5-(trifluoromethyl)-2,3-dihydro-1~{H}-1,4-diazepine 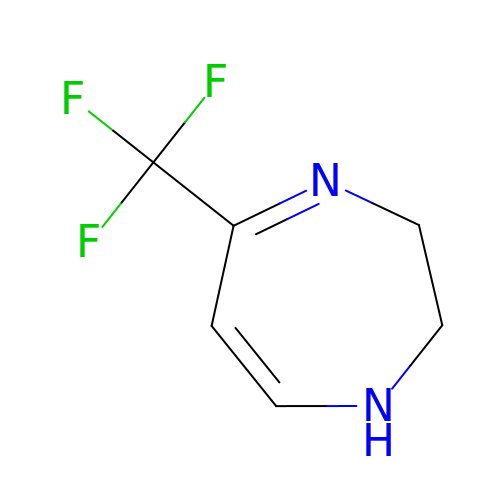| C6 H7 F3 N2 | DQLAMAHCMYJIBW-UHFFFAOYSA-N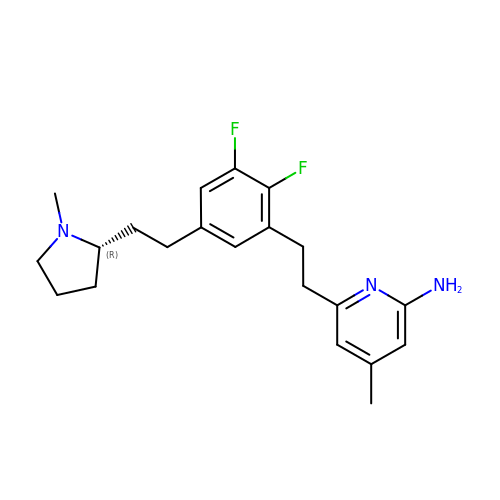6-[2-(2,3-difluoro-5-{2-[(2R)-1-methylpyrrolidin-2-yl]ethyl}phenyl)ethyl]-4-methylpyridin-2-amine | C21 H27 F2 N3 | DWIFPRVVASXUJK-SFHVURJKSA-N>SNAMNSQLTLRALERGDLRFIHNLNNNRNIMSYWFEEPYESFDELEELYNKHIHDNAERRFVVEDAQKNLIGLVELIEINYIHRSAEFQI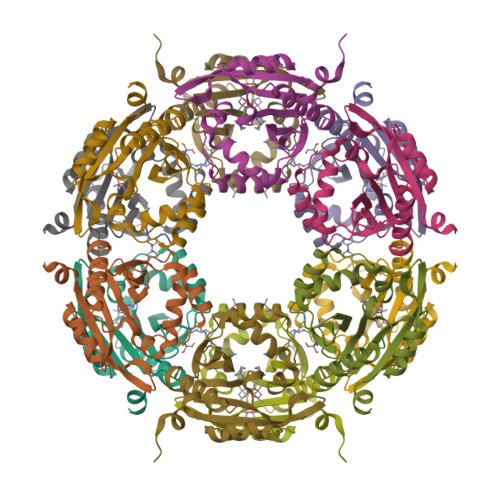IIAPEHQGKGFARTLINRALDYSFTILNLHKIYLHVAVENPKAVHLYEECGFVEEGHLVEEFFINGRYQDVKRMYILQSKYLNRSE[6x]>MHHHHHHENLYFQSTKASLTYSQLSKEIANNIDTMAKALTTMQEQIDSLAAVVLQNRRGLDMLTAAQGGICLALDEKCCFWVNQSGKVQDNIRQLLN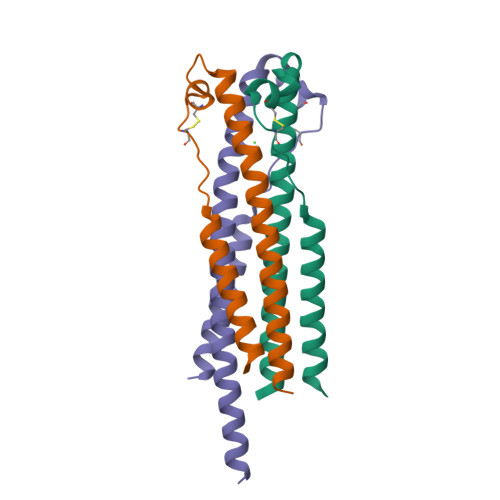QASSLRERATQ[3x]> VDCSEYPKPACTWEYRPLCGSDNKTYGNKCNFCNAVV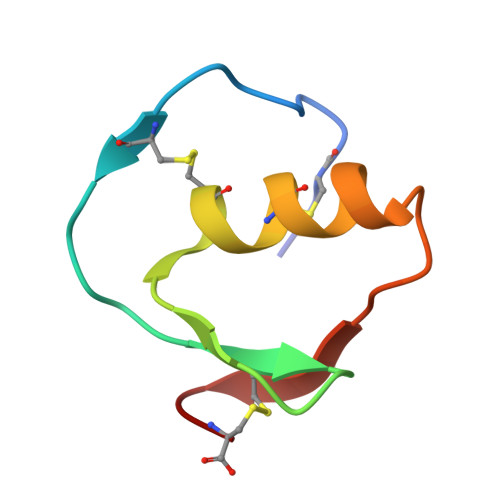ESNGTLTLSHFGKC> MASWSHPQFEKGASLDSPTFGCTDSPVRRERGQKAVFCGLTSIVWLHRKMQDAFFLVVGSRTCAHLLQAAAGVMIFAEPRFGTAVLEEQDLAG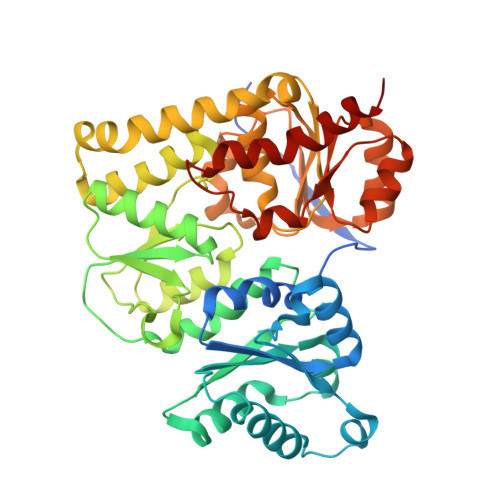LADAHKELDREVAKLLERRPDIRQLFLVGSCPSEVLKLDLDRAAERLSGLHAPHVRVYSYTGSGLDTTFTQGEDTCLAAMVPTLDTTEAAELIVVGALPDVVEDQCLSLLTQLGVGPVRMLPARRSDIEPAVGPNTRFILAQPFLGETTGALERRGAKRIAAPFPFGEEGTTLWLKAVADAYGVSAEKFEAVTAAPRARAKKAIAAHLETLTGKSLFMFPDSQLEIPLARFLARECGMKTTEIATPFLHKAIMAPDLALLPSNTALTEGQDLEAQLDRHEAINPDLTVCGLGLANPLEAKGHATKWAIELVFTPVHFYEQAGDLAGLFSRPLRRRALLNGGAA>MTDSSSLRGVDADTEKRINVGKTHLQTLRNLETRCHDSLQALVVIDAGSSSTRTNVFLAKTRSCPNKGRSIDPDSIQLIREGKRFTGLRVVLEEWLDTYAGKDWESRPVDARLLFQYVPQMHEGAKKLMQLLEEDTVAILDSQLNEEQKVQVKALGIPVMLCSTAGVRDFHEWYRDALFVLLRHLINNPSPAHGYKFFTNPFWTRPITGAEEGLFAFITLNHLSRRLGEDPARCMIDEYGVKHCRNDLAGVVEVGGASAQIVFPLQEGTVLPSSVRAVNLQRERLLPERYPSADVVSVSFMQLGMASSAGLFLKELCSNDEFLQGGICSNPCLFKGFQQSCSAGEVEVRPDGSASVNEDVRKNRLKPLATYCSVHNPEISFKVTNEMQCRENSIDPTKPLAERMKIENCSIIEGTGNFDKCVSQVESILVAPKLPLPANIEAASSGFESVDQVFRFA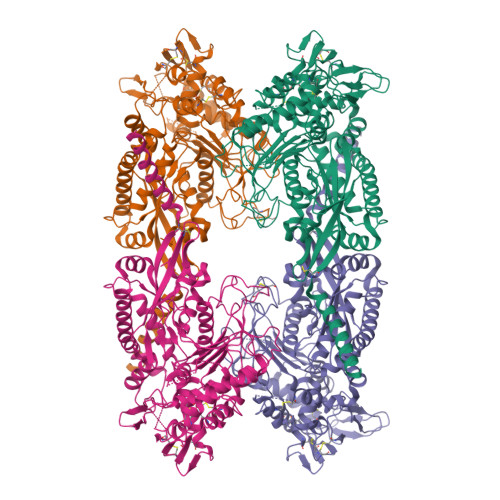SSTAPMFITGREMLASIDTLKDHRLLRSDFSGDVEELAEAAREFCSSEVIIRTDGPVIQLPNARGEQKLNSLNFDLCKTMALTVSLLRHMAAGENQPSFIKWEKSIAGPDGKPLADLGWQVGVILHHVLFTEEWGRTAYEAGYSHNLEHHHHHH[2x]>[24x]SMQRTVARQVALVECVGKGRYGEVWRGLWHGESVAVKIFSSRDEQSWFRETEIYNTVLL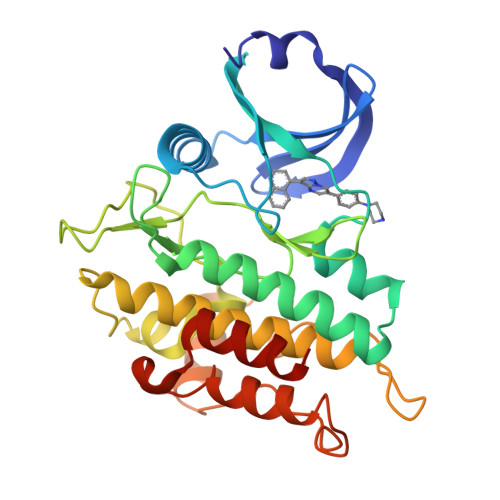RHDNILGFIASDMTSRNSSTQLWLITHYHEHGSLYDFLQRQTLEPHLALRLAVSAACGLAHLHVEIFGTQGKPAIAHRDFKSRNVLVKSNLQCCIADLGLAVMHSQGSDYLDIGNNPRVGTKRYMAPEVLDEQIRTDCFESYKWTDIWAFGLVLWEIARRTIVNGIVEDYRPPFYDVVPNDPSFEDMKKVVCVDQQTPTIPNRLAADPVLSGLAQMMRECWYPNPSARLTALRIKKTLQKISNSPE>GSGGRATMEPSALRKAGSEQEEGFEGLPRRVTDLGMVSNLRRSNSSLFKSWRLQCPFGNNDKQESLSSWIPENIKKKECVYFVESSKLSDAGKVVCQCGYTHEQHLEEATKPHTFQGTQWDPKKHVQEMPTDAFGDIVFTGLSQKVKKYVRVSQDTPSSVIYHLMTQHWGLDVPNLLISVTGGAKNFNMKPRLKSIFRRGLVKVAQTTGAWIITGGSHTGVMKQVGEAVRDFSLSSSYKEGELITIGVATWGTVHRREGLIHPTGSFPAEYILDEDGQGNLTCLDSNHSHFILVDDGTHGQYGVEIPLRTRLEKFISEQTKERGGVAIKIPIVCVVLEGGPGTLHTIDNATTNGTPCVVVEGSGRVADVIAQVANLPVSDITISLIQQKLSVFFQEMFETFTESRIVEWTKKIQDIVRRRQLLTVFREGKDGQQDVDVAILQALLKASRSQDHFGHENWDHQLKLAVAWNRVDIARSEIFMDEWQWKPSDLHPTMTAALISNKPEFVKLFLENGVQLKEFVTWDTLLYLYENLDPSCLFHSKLQKVLVEDPERPACAPAAPRLQMHHVAQVLRELLGDFTQPLYPRPRHNDRLRLLLPVPHVKLNVQGVSLRSLYKRSSGHVTFTMDPIRDLLIWAIVQNRRELAGIIWAQSQDCIAAALACSKILKELSKEEEDTDSSEEMLALAEEYEHRAIGVFTECYRKDEERAQKLLTRVSEAWGKTTCLQLALEAKDMKFVSHGGIQAFLTKVWWGQLSVDNGLWRVTLCMLAFPLLLTGLISFREKRLQDVGTPAARARAFFTAPVVVFHLNILSYFAFLCLFAYVLMVDFQPVPSWCECAIYLWLFSLVCEEMRQLFYDPDECGLMKKAALYFSDFWNKLDVGAILLFVAGLTCRLIPATLYPGRVILSLDFILFCLRLMHIFTISKTLGPKIIIVKRMMKDVFFFLFLLAVWVVSFGVAKQAILIHNERRVDWLFRGAVYHSYLTIFGQIPGYIDGVNFNPEHCSPNGTDPYKPKCPESDATQQRPAFPEWLTVLLLCLYLLFTNILLLNLLIAMFNYTFQQVQEHTDQIWKFQRHDLIEEYHGRPAAPPPFILLSHLQLFIKRVVLKTPAKRHKQLKNKLEKNEEAALLSWEIYLKENYLQNRQFQQKQRPEQKIEDISNKVDAMVDLLDLDPLKRSGSMEQRLASLEEQVAQTAQALHWIVRTLRASGFSSEADVPTLASQKAAEEPDAEPGGRKKTEEPGDSYHVNARHLLYPNCPVTRFPVPNEKVPWETEFLIYDPPFYTAERKDAAAMDPMGDTLEPLSTIQYNVVDGLRDRRSFHGPYTVQAGLPLNPMGRTGLRGRGSLSCFGPNHTLYPMVTRWRRNEDGAICRKSIKKMLEVLVVKLPLSEHWALPGGSREPGEMLPRKLKRILRQEHWPSFENLLKCGMEVYKGYMDDPRNTDNAWIETVAVSVHFQDQNDVELNRLNSNLHACDSGASIRWQVVDRRIPLYANHKTLLQKAAAEFGAHYFE[4x]

Intracellular ADPR targets and activates the nonselective, calcium-permeable TRPM2 channel in the presence of Ca2+. Belonging to the transient receptor potential melastatin family (TRPM), TRPM2 shares a characteristic MHR1-4 domain, a transmembrane domain (TMD), and a coiled-coil domain with the other family members. It is unique due to owning a characteristic C-terminal NUDT9-H domain, which has been considered a classic binding site for ADPR and its derivatives, but the presence of the ADPR binding site has not been directly observed. In summary, our human TRPM2 structures defined two distinctive ADPR binding sites, one in the MHR1/2 domain and one in the NUDT9-H domain.

In both ADPR-bound structures, ADPR densities were observed in two different sites on each subunit, one (ADPR1) in the cleft of the MHR1/2 domain and a second (ADPR2) in the cleft of the NUDT9-H domain. Relative to the apo state, the binding of ADPR to hsTRPM2 yielded a markedly elevated MHR1/2 layer and a contracted NUDT9-H layer, with the NUDT9-H domain swinging toward the pore axis. Therefore, ADPR1 is bent into a compact U shape to adapt to the MHR1/2 site, similar to the finding in the drTRPM2 structure. ADPR1 is clamped between Y295 and the loop connecting the β5 strand α3 helix (β5-α3 loop), with the terminal adenine and terminal ribose moieties close to each other. In contrast, the cleft in the NUDT9-H domain is wider, embraced by its cap and core regions on each side and the central β sheet on the bottom, allowing ADPR2 to nestle in an extended shape with the terminal adenine and terminal ribose moieties far apart. The adenine moiety of ADPR2 stacks between Y1485 and D1431, while the α-phosphate group interacts with R1433. ADPR binding into the cleft of MHR1/2 led to a clamshell closure similar to that observed in the drTRPM2 structures. Binding of ADPR into the cleft of the NUDT9-H induced a rigid-body rotation of the core region toward the cap region, resulting in a bi-lobed domain closure. Within the TMD specifically, although the pore domain showed little change, the S1-S4 domain underwent a remarkable clockwise rotation around the pore axis. Because ADPR alone cannot active the TRPM2 channel in the absence of Ca2+, we designated the ADPR-hsTRPM2 structure as a ADPR-bound non-activated state.> XXXXXXXXXXXXXXXXXXXXXXXXXXXXXXXXXXXXXXXXXXXXXXXXXXXXXXXXXXXXXXXXXXXXXXXXXXXXXXXXXXXXXXXXXXXXXXXXXXXXXXXXXXXXXXXXXXXXXXXXXXXXXXXXXXXXXXXXXXXXXXXXXXXXXXXXXXXXXXXXXXXXXXXXXXXXXXXXXXXXXXXXXXXXXXXXXXXXXXXXXXXXXXXXXXXXXXXXXXXXXXXXXXXXXXXXXXXXXXXXXXXXXXXXXXXXXXXXXXXXXXXXXXXXXXXXXXXXXXXXXXXXXXXXXXXXXXXXXXXXXXXXXXFSTNFRDTVDILVGWHIDHTQKPSLTQQVSGWLQSLEPFWVADLAFSTTLLGQFLEDMEAYAEDLSHVASGESVDEDVPPPSVSLPKLAALLRVFSTVVRSIGERFSPIRGPPITEAYVTDVLYRVMRCVTAANQVFFSEAVLTAANECVGVLLGSLDPSMTIHCDMVITYGLDQLENCQTCGTDYIISVLNLLTLIVEQINTKLPSSFVEKLFIPSSKLLFLRYHKEKEVVAVAHAVYQAVLSLKNIPVLETAYKLILGEMTCALNNLLHSLQLPEACSEIKHEAFKNHVFNVDNAKFVVIFDLSALTTIGNAKNSLIGMWALSPTVFALLSKNLMIVHSDLAVHFPAIQYAVLYTLYSHCTRHDHFISSSLSSSSPSLFDGAVISTVTTATKKHFSIILNLLGILLKKDNLNQDTRKLLMTWALEAAVLMRKSETYAPLFSLPSFHKFCKGLLANTLVEDVNICLQACSSLHALSSSLPDDLLQRCVDVCRVQLVHSGTRIRQAFGKLLKSIPLDVVLSNNNHTEIQEISLALRSHMSKAPSNTFHPQDFSDVISFILYGNSHRTGKDNWLERLFYSCQRLDKRDQSTIPRNLLKTDAVLWQWAIWEAAQFTVLSKLRTPLGRAQDTFQTIEGIIRSLAAHT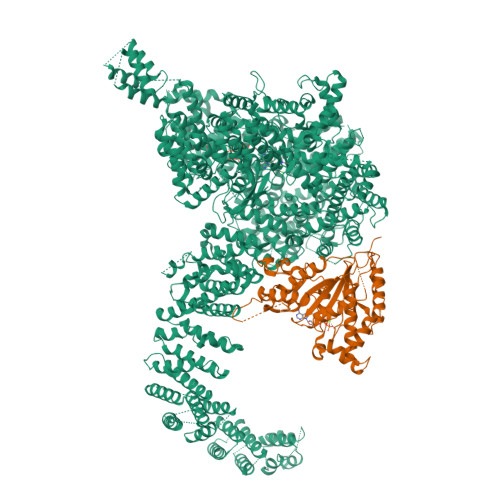LNPDQDVSQWTTADNDEGHGNNQLRLVLLLQYLENLEKLMYNAYEGCANALTSPPKVIRTFFYTNRQTCQDWLTRIRLSIMRVGLLAGQPAVTVRHGFDLLTEMKTTSLSQGNELEVTIMMVVEALCELHCPEAIQGIAVWSSSIVGKNLLWINSVAQQAEGRFEKASVEYQEHLCAMTGVDCCISSFDKSVLTLANAGRNSASPKHSLNGESRKTVLSKPTDSSPEVINYLGNKACECYISIADWAAVQEWQNSIHDLKKSTSSTSLNLKADFNYIKSLSSFESGKFVECTEQLELLPGENINLLAGGSKEKIDMKKLLPNMLSPDPRELQKSIEVQLLRSSVCLATALNPIEQDQKWQSITENVVKYLKQTSRIAIGPLRLSTLTVSQSLPVLSTLQLYCSSALENTVSNRLSTEDCLIPLFSEALRSCKQHDVRPWMQALRYTMYQNQLLEKIKEQTVPIRSHLMELGLTAAKFARKRGNVSLATRLLAQCSEVQLGKTTTAQDLVQHFKKLSTQGQVDEKWGPELDIEKTKLLYTAGQSTHAMEMLSSCAISFCKSVKAEYAVAKSILTLAKWIQAEWKEISGQLKQVYRAQHQQNFTGLSTLSKNILTLIELPSVNTMEEEYPRIESESTVHIGVGEPDFILGQLYHLSSVQAPEVAKSWAALASWAYRWGRKVVDNASXXXXXXXXXXXXXXXXXXXXXXXXXXXXXXXXXXXXXXXXXXXXXXXXXXXXXXXXXXXXXXXXXXXXXXXXXXXXXXXXXXXXXXXXEGVIKVWRKVVDRIFSLYKLSCSAYFTFLKLNAGQIPLDEDDPRLHLSHRVEQSTDDMIVMATLRLLRLLVKHAGELRQYLEHGLETTPTAPWRGIIPQLFSRLNHPEVYVRQSICNLLCRVAQDSPHLILYPAIVGTISLSSESQASGNKFSTAIPTLLGNIQGEELLVSECEGGSPPASQDSNKDEPKSGLNEDQAMMQDCYSKIVDKLSSANPTMVLQVQMLVAELRRVTVLWDELWLGVLLQQHMYVLXXXXXXXXXXXXXXXXXXXXXXXXXXXXXXXXXXXXXXXXXXXXXXXXXXXXXXXXPHEKWFQDNYGDAIENALEKLKXXXXXXXXXXXXXXXXXXXXXXXXXXXXXXXYILRLEEISPWLAAMTNTEIALPGEVSARDTVTIHSVGGTITILPTKTKPKKLLFLGSDGKSYPYLFKGLEDLHLDERIMQFLSIVNTMFATINRQETPRFHARHYSVTPLGTRSGLIQWVDGATPLFGLYKRWQQREAALQAQKAQDSYQTPQNPGIVPRPSELYYSKIGPALKTVGLSLDVSRRDWPLHVMKAVLEELMEATPPNLLAKELWSSCTTPDEWWRVTQSYARSTAVMSMVGYIIGLGDRHLDNVLIDMTTGEVVHIDYNVCFEKGKSLRVPEKVPFRMTQNIETALGVTGVEGVFRLSCEQVLHIMRRGRETLLTLLEAFVYDPLVDWTAGGEAGFAGAVYGGGGQQAESKQSKREMEREITRSLFSSRVAEIKVNWFKNRDEMLVVLPKLDGSLDEYLSLQEQLTDVEKLQGKLLEEIEFLEGAEGVDHPSHTLQHRYSEHTQLQTQQRAVQEAIQVKLNEFEQWITHYQAAFNNLEATQLASLLQEISTQMDLGPPSYVPATAFLQNAGQAHLISQCEQLEGEVGALLQQRRSVLRGCLEQLHHYATVALQYPKAIFQKHRIEQWKTWMEELICNTTVERCQELYRKYEMQYAPQPPPTVCQFITATEMTLQRYAADINSRLIRQVERLKQEAVTVPVCEDQLKEIERCIKVFLHENGEEGSLSLASVIISALCTLTRRNLMMEGAASSAGEQLVDLTSRDGAWFLEELCSMSGNVTCLVQLLKQCHLVPQDLDIPNPMEASETVHLANGVYTSLQELNSNFRQIIFPEALRCLMKGEYTLESMLHELDGLIEQTTDGVPLQTLVESLQAYLRNAAMGLEEETHAHYIDVARLLHAQYGELIQPRNGSVDETPKMSAGQMLLVAFDGMFAQVETAFSLLVEKLNKMEIPIAWRKIDIIREARSTQVNFFDDDNHRQVLEEIFFLKRLQTIKEFFRLCGTFSKTLSGSSSLEDQNTVNGPVQIVNVKTLFRNSCFSEDQMAKPIKAFTADFVRQLLIGLPNQALGLTLCSFISALGVDIIAQVEAKDFGAESKVSVDDLCKKAVEHNIQIGKFSQLVMNRATVLASSYDTAWKKHDLVRRLETSISSCKTSLQRVQLHIAMFQWQHEDLLINRPQAMSVTPPPRSAILTSMKKKLHTLSQIETSIATVQEKLAALESSIEQRLKWAGGANPALAPVLQDFEATIAERRNLVLKESQRASQVTFLCSNIIHFESLRTRTAEALNLDAALFELIKRCQQMCSFASQFNSSVSELELRLLQRVDTGLEHPIGSSEWLLSAHKQLTQDMSTQRAIQTEKEQQIETVCETIQNLVDNIKTVLTGHNRQLGDVKHLLKAMAKDEEAALADGEDVPYENSVRQFLGEYKSWQDNIQTVLFTLVQAMGQVRSQEHVEMLQEITPTLKELKTQSQSIYNNLVSFASPLVTDATNECSSPTSSATYQPSFAAAVRSNTGQKTQPDVMSQNARKLIQKNLATSADTPPSTVPGTGKSVACSPKKAVRDPKTGKAVQERNSYAVSVWKRVKAKLEGRDVDPNRRMSVAEQVDYVIKEATNLDNLAQLYEGWTAWV;> MSESGHSQPGLYGIERRRRWKEPGSGGPQNLSGPGGRERDYIAPWERERRDASEETSTSVMQKTPIILSKPPAERSKQPPPPTAPAAPPAPAPLEKPIVLMKPREEGKGPVAVTGASTPEGTAPPPPAAPAPPKGEKEGQRPTQPVYQIQNRGMGTAAPAAMDPVVGQAKLLPPERMKHSIKLVDDQMNWCDSAIEYLLDQTDVLVVGVLGLQGTGKSMVMSLLSANTPEEDQRTYVFRAQSAEMKERGGNQTSGIDFFITQERIVFLDTQPILSPSILDHLINNDRKLPPEYNLPHTYVEMQSLQIAAFLFTVCHVVIVVQDWFTDLSLYRFLQTAEMVKPSTPSPSHESSSSSGSDEGTEYYPHLVFLQNKARREDFCPRKLRQMHLMIDQLMAHSHLRYKGTLSMLQCNVFPGLPPDFLDSEVNLFLVPFMDSEAESENPPRAGPGSSPLFSLLPGYRGHPSFQSLVSKLRSQVMSMARPQLSHTILTEKNWFHYAARIWDGVRKSSALAEYSRLLA> MTERLNEQNNESYRYLRSVGNQWQFNVEDLHPKMLSRLYKRFDTFDLDSDGKMEMDEVLYWPDRMRQLVNATDEQVEKMRDAVRVFFLHKGVEPVNGLLREDWVEANRVFAEAERERERRGEPSLIALLSNSYYDVLDDDGDGTVDVDELKTMMKAFDVPQEAAYTFFEKADTDKSGKLERTELVHLFRKFWMEPYDPQ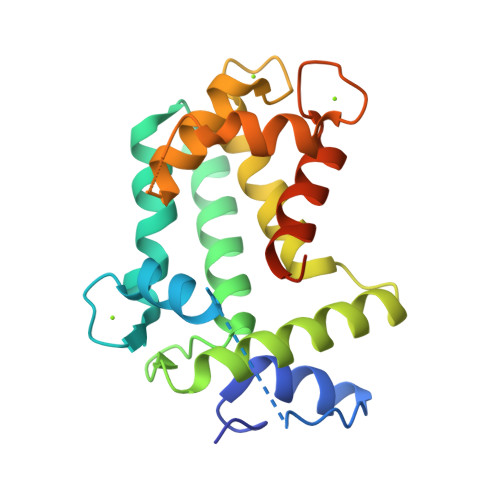WDGVYAYKY>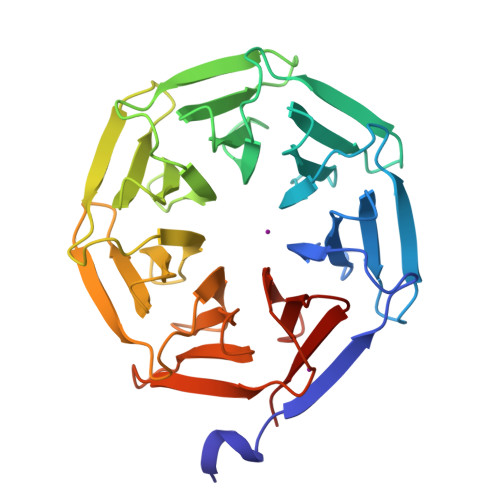 GSEAWMNFYLEEFNLSIPDSGPYGITSSEDGKVWFTQHKANKISSLDQSGRIKEFEVPTPDAKVMCLIVSSLGDIWFTENGANKIGKLSKKGGFTEYPLPQPDSGPYGITEGLNGDIWFTQLNGDRIGKLTADGTIYEYDLPNKGSYPAFITLGSDNALWFTENQNNSIGRITNTGKLEEYPLPTNAAAPVGITSGNDGALWFVEIMGNKIGRITTTGEISEYDIPTPNARPHAITAGKNSEIWFTEWGANQIGRITNDNTIQEYQLQTENAEPHGITFGKDGSVWFALKCKIGKLNLNE> MITMKDIIREGNPTLRAVAEEVPVPITEEDRQLGEDMLTFLKNSQDPVKAEELQLRGDVGLAAPQLDISKRIIAVHVPSNDPENETPSLSTVMYNPKILSHSVQDVCLGEGEGCLSVDRDVPGYVVRHNKITVSYFDMAGEKHKVRLKNYEAIVVQHEIDHINGIMFYDHINKEN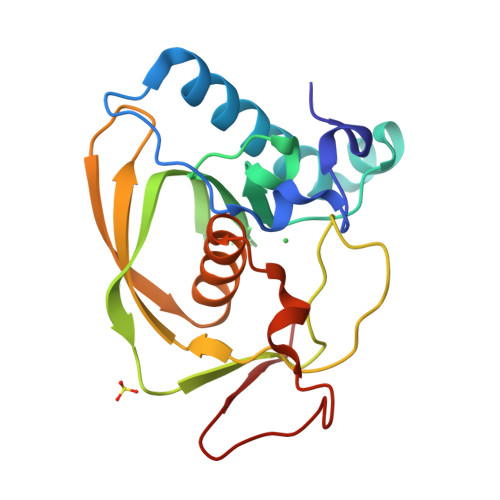PFALKEGVLVIEL> GDIVSEKKPATEVDPTHFEKRFLKRIRDLGEGHFGKVELCRYDPEGDNTGEQVAVKSLKPESGGNHIADLKKEIEILRNLYHENIVKYKGICTEDGGNGIKLIMEFLPSGSLKEYLPKNKNKINLKQQLKYAVQICKGMDYLGSRQYVHRDLAARNVLVESEHQVKIGDFGLTKAIETDKEYYTVKDDRDSPVFWYAPECLMQSKFYIASDVWSFGVTLHELLTYCDSDSSPMALFLKMIGPTHGQMTVTRLVNTLKEGKRLPCPPNCPDEVYQLMRKCWEFQPSNRTSFQNLIEGFEALLK;> DIVSEKKPATEVDPTHFEKRFLKRIRDLGEGHFGKVELCRYDPEGDNTGEQVAVKSLKPESGGNHIADLKKEIEILRNLYHENIVKYKGICTEDGGNGIKLIMEFLPSGSLKEYLPKNKNKINLKQQLKYAVQICKGMDYLGSRQYVHRDLAARNVLVESEHQVKIGDFGLTKAIETDKEYYTVKDDRDSPVFWYAPECLMQSKFYIASDVWSFGVTLHELLTYCDSDSSPMALFLKMIGPTHGQMTVTRLVNTLKEGKRLPCPPNCPDEVYQLMRKCWEFQPSNRTSF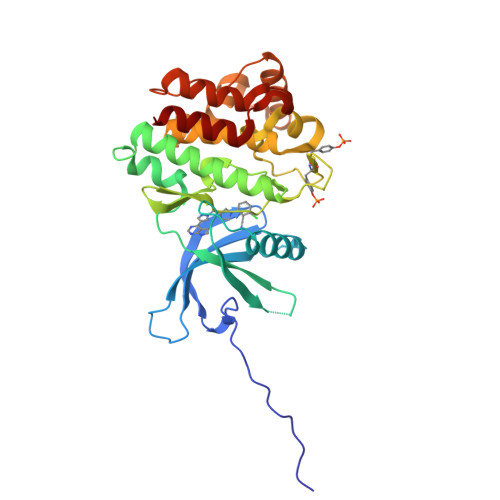QNLIEGFEALLK Insects, instead, rely on a distinct family of sweet gustatory receptors, which are tetrameric ligand-gated cation channels. An extreme example of sugar specialization occurs in a conserved subfamily of gustatory receptors founded by Drosophila melanogaster Gr43a (DmGr43a), whose members are selectively activated only by the monosaccharide d-fructose, providing a unique opportunity to investigate how specificity for a single sugar is achieved. Here we investigate the structural basis of sugar discrimination by Gr9 (BmGr9), the silk moth B. mori orthologue of DmGr43a. Our results thus indicate that receptor tuning in BmGr9 arises from two distinct but complementary mechanisms: the stereoelectronic characteristics of the ligand-binding pocket; and the engagement of an allosteric process required to activate the channel.

Consistent with our docking results, our data show that l-sorbose binds BmGr9 with an affinity close to that of d-fructose whereas sucrose did not induce a shift in the tryptophan fluorescence spectrum. We therefore determined the structure of BmGr9 in a third gating state bound to a non-activating sugar, l-sorbose, but with a closed pore. As other hexoses are predicted to make many of the same contacts as d-fructose, it is unclear why they do not activate BmGr9. d-Fructose and l-sorbose differ by the chirality of a single hydroxyl group at the C5 position. In l-sorbose, the inverted stereochemistry of C5 places a hydroxyl group in the middle of the hydrophobic patch, probably impeding proper engagement of the aromatic bridge and preventing binding being transduced to pore opening. To test our hypothesis, we determined the structure of BmGr9 in the presence of a saturating amount of l-sorbose to a nominal resolution of 2.6 Å. l-Sorbose exists predominantly in a six-membered ring conformation (about 98% α-l-sorbopyranose), whose single hydroxymethyl arm matches the asymmetric density for the bound ligand well. In the pocket, l-sorbose makes many of the same interactions as d-fructose: a hydrophobic surface (hydrogens of C1 and C3) faces Trp354 and the hydroxyl groups are all coordinated. However, l-sorbose does not interact with Phe333 of the aromatic bridge; therefore, there is no link between l-sorbose in the binding pocket and the pore helix, leaving the ion-conducting pore in a closed conformation. This structure, with a bound ligand but closed pore, illustrates how the structural changes associated with ligand binding may be uncoupled from those leading to channel activation. Indeed, our structure of BmGr9 bound to l-sorbose reveals that non-activating sugars not only can fit into the ligand-binding pocket, but also can make many of the same contacts as d-fructose, yet the pore is closed.

>GPGRAPPSPDLRADEPKTPCLVGGAHAFILKISSFCGLAPLRFEPRSQEYAVTISKGKCFYSYILVTFLVICTIYGLVAEIGVGVEKSVRMSSRMSQVVSACDILVVAVTAGVGVYGAPARMRTMLSYMENIVAVDRELGRHHSAATERKLCALLLLILLSFTILLVDDFCFYAMQAGKTGRQWEIVTNYAGFYFLWYIVMVLELQFAFTALSLRARLKLFNEALNVTASQVCKPVKKPKNSQLSVYATSVRPVSCKRENVIVETIRVRDKDDAFVMMKTADGVPCLQVPPCEAVGRLSRMRCTLCEVTRHIADGYGLPLVIILMSTLLHLIVTPYFLIMEIIVSTHRLHFLVLQFLWCTTHLIRMLVVVEPCHYTIREGKRTEDILCRLMTLAPHGGVLSSRLEVLSRLLMLQNISYSPLGMCTLDRPLMVTVLGAVTTYLVILIQFQRYDS[4x]>[3x]FACKTANGTAIPIGGGSANVYVNLAPVVNVGQNLVVDLSTQIFCHNDYPETITDYVTLQRGSAYGGVLSNFSGTVKYSGSSYP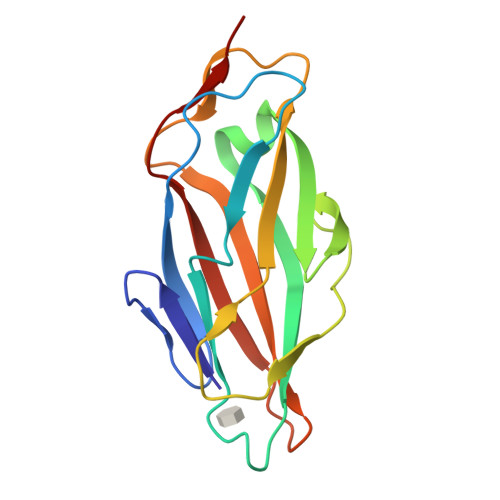FPTTSETPRVVYNSRTDKPWPVALYLTPVSSAGGVAIKAGSLIAVLILRQTNNYNSDDFQFVWNIYANNDVVVPT> ARTVVLITGCSSGIGLHLAVRLASDPSQSFKVYATLRDLKTQGRLWEAARALACPPG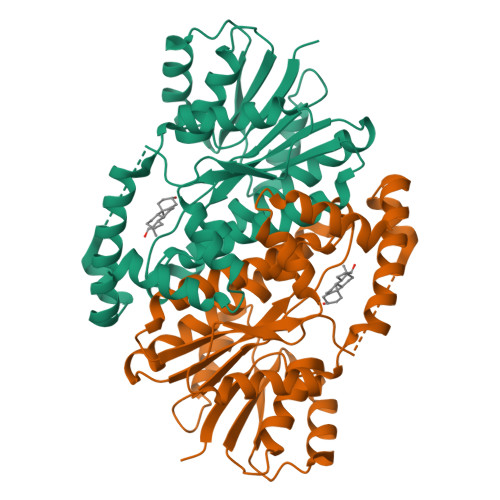SLETLQLDVRDSKSVAAARERVTEGRVDVLVCNAGLGLLGPLEALGEDAVASVLDVNVVGTVRMLQAFLPDMKRRGSGRVLVTGSVGGLMGLPFNDVYCASKFALEGLCESLAVLLLPFGVHLSLIECGPVHTAFMEKVLGSPEEVLDRTDIHTFHRFYQYLAHSKQVFREAAQNPEEVAEVFLTALRAPKPTLRYFTTERFLPLLRMRLDDPSGSNYVTAMHREVFGDVPAKAEAGAEAGGGAGPGAEDEAGRSAVGDPELGDPPAAPQ N-[(4-PHENYL-1H-1,2,3-TRIAZOL-1-YL)ACETYL]-BETA-D-GLUCOPYRANOSYLAMINE 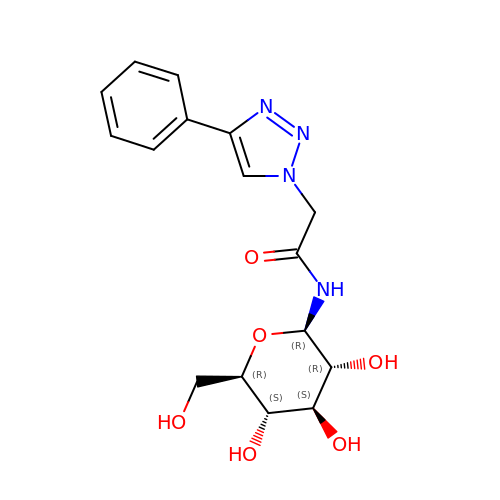| C16 H20 N4 O6 | NWFJPPOXTYDHDB-YMILTQATSA-N> GAACGACACTGA;> CGGCGACTC;> TCACCG;> TCGAGTCGGTGTCGT

In this work, we exhaustively probe the ability of all 36 immobile HJ sequences to form DNA crystals in two different designed systems. Three separate self-assembling DNA crystal systems are described in this report: the “4 × 5” and “4 × 6” designs (collectively referred to as the 4 × N systems), and a third construct with a “scrambled” sequence variant of the 4 × 6 lattices. Self-assembly was mediated by three constituent oligonucleotides: (S1) containing four sequence repeats of either 5 or 6 bases; (S2) composed of 21 bases containing complementary regions to both (S1); and (S3) which forms the second junction crossover. The HJ serves as the fundamental component at the core of each unit, and the ultimate assembly of the full lattice is facilitated by the complementary 2-base sticky ends that tail each duplex.

To investigate this possibility, we designed “scrambled” sequences with targeted base substitutions, while maintaining GC content, along each “stem”. Contrary to the buffer preference observed with the native P32 crystals, the scrambled systems exhibited an exclusive preference towards low salt buffers, much like the native R3 crystals. Remarkably, only J1 and J2 retained the P32 symmetry, with all others yielding an R3 lattice. There appeared to be only a marginal difference in the average cell lengths in the R3 scramble crystals (a = b = 113.04 c = 51.10) relative to the native 4 × 6 sequences: the a, b axis trended ~2 Å shorter and c ~1.3 Å longer, whereas in the J1 and J2 cases, the crystals were in good agreement with the original 4 × 6 motif. The average angles of the R3 and P32 crystals were 61.00° (σ = 1.21) and 58.05° (σ = 1.39), respectively. The role of longer-range sequence effects on junction angles remains a largely open question, but the effect in our crystal system is significant. However, in the majority of the crystal structures reported here, the cacodylate anion indeed fits best into the electron density map of our X-ray structures, due to the presence of sodium cacodylate in the crystallization solution.>MPVFHTRTIESILEPVAQQISHLVIMHEEGEVDGKAIPDLTAPVAAVQAAVSNLVRVGKETVQTTEDQILKRDMPPAFIKVENACTKLVQAAQMLQSDPYSVPARDYLIDGSRGILSGTSDLLLTFDEAEVRKIIRVCKGILEYLTVAEVVETMEDLVTYTKNLGPGM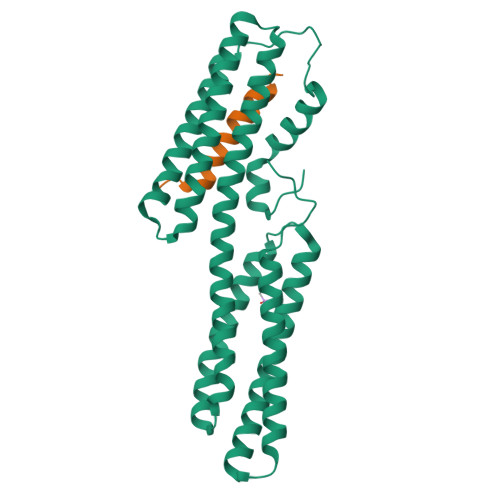TKMAKMIDERQQELTHQEHRVMLVNSMNTVKELLPVLISAMKIFVTTKNSKNQGIEEALKNRNFTVEKMSAEINEIIRVLQLTSWDEDAW[2x];>GSHMTRETIFEASKKVTNSLSNLISLIGT[2x]> MGSDKIHHHHHHMAFTPFPPRQPTASARLPLTLMTLDDWALATITGADSEKYMQGQVTADVSQMAEDQHLLAAHCDAKGKM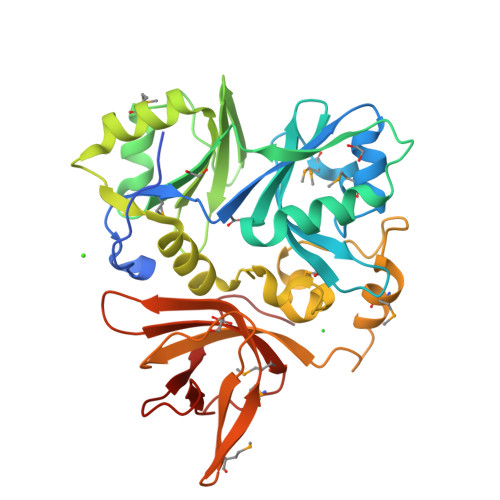WSNLRLFRDGDGFAWIERRSVREPQLTELKKYAVFSKVTIAPDDERVLLGVAGFQARAALANLFSELPSKEKQVVKEGATTLLWFEHPAERFLIVTDEATANMLTDKLRGEAELNNSQQWLALNIEAGFPVIDAANSGQFIPQATNLQALGGISFKKGCYTGQEMVARAKFRGANKRALWLLAGSASRLPEAGEDLELKMGENWRRTGTVLAAVKLEDGQVVVQVVMNNDMEPDSIFRVRDDANTLHIEPLPYSLEE>[4x]GGPIPYPVGNLLHTAPCGFIVTDAVEPDQPIIYVNTVFEMVTGYRAEEVLGR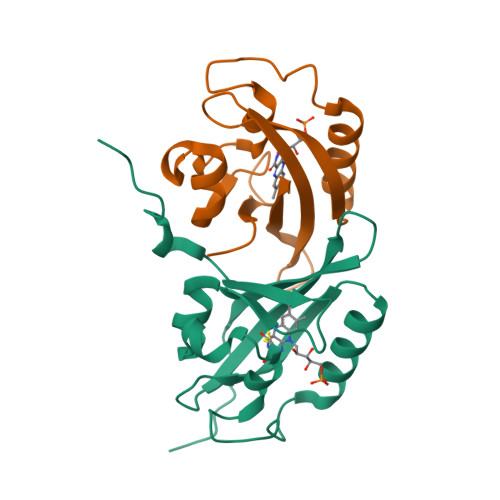NCRFLQCRGPFAKRRHPLVDSMVVSEIRKCIDEGIEFQGELLNFRKDGSPLMNRLRLTPIYGDDDTITHIIGIQFFIETDIDLGP> SNAMISKLSVNPTFSPSYNIIVDSVLDFSHILEYVTNKQVLVVTNTTVAKLYLTKFLAALVDDLDVRTCILEDGEQYKSQQSLDKILSTLLENHFTRNSTVL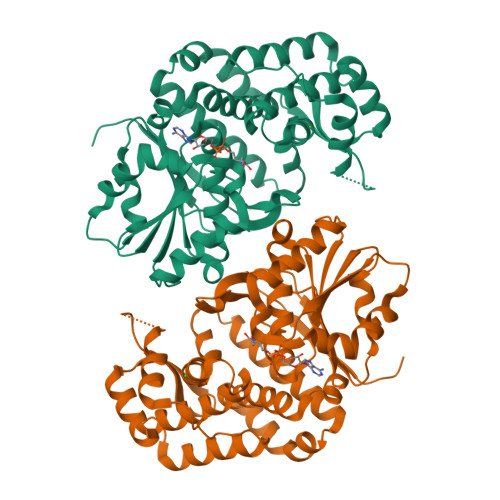VALGGGVIGDITGFAAAIYQRGIDFIQIPTTLLSQVDSSVGGKTAINHQLGKNMIGAFYQPKVVYTSIEFYKTLPQREYIAGMAEVVKYAFISKDFYLWLDSNRDKILAKDSVTLIEMVKRSCQIKAQVVAMDEKELTGARAILNFGHTFGHAIEKCQNYRGLKHGEAVGVGMAQAIDFSHYLGLISQQQAKDFNDFIVSFGISIDFPNDICQKEFLEAMLLDKKNSNKELKFILIENIGSLSLQKQSKNELEQFLDISR> MAPTPKYTFTERAAAGNLSDAEILNSNNPTGSELPDESDVVVGGAGIHGLIYALHASKYKPNNLKISVIEKNTRPGYKIGESTLPIFYTWCKLHGI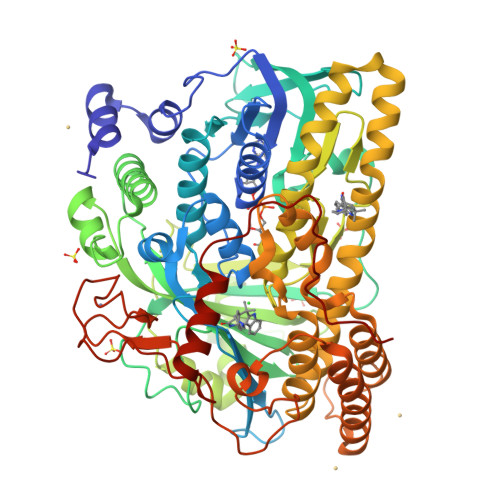SAAYLLRLFGLKDGLSFYFLDRENQGQYTDFSSVGAPGLVLASLQIERPMSELLFTILAQRNGVNVYHGREVDFKSTVVQGGGQGNKIAVSRGKYDSTPKTIDSALFVDATGRFRQFCSKKAPRHRFDGWNCNAFWGYFTAPKDESKIPFDLYEGDHTNHLCFPEGWVWVIRLPSWEGSPIANLMDMVTYILECADAGVPGDELPSSEELARMFGLKFQWVTSIGFAVRNDVKYPEDLSAYGTREAEQKFNYFVQKYELLQQFMSNFELIENLYGPGTTWFIRKTLAYQSPVVSGPGWLAIGDACGFTNPLYSPGINVGMSTSTWAAQLSHPIVEIGKSAPADAAESSIRKLLVPYDDYCKSLVPALEQMNRFNYVCYRDTRLGPQVACLWQFFAGIERYLSDVNIETFAHYAIKWVWGAMVPEYQQVAQKCIEHIETVPLDERLPDAMVDELLAFSNRIKSAAVAADDFSLRWDAILRSFDRSLNFVEGKTSRDIYTRQCSGCGAWLQLRPDWKKCHSCGLLGTEPQTAVTFDPPLTAEEEALLYAAWNTAPKYDPSKELKLPTPTRPAA>MNQETLIAVVEQMRKLVPALRKVPDETLYAWVEMAELFVCQKTFKDAYVKALALYALHLAFLDGALKGEDEDLESYSRRVTSFSLSGEFSQTFGEVTKNQSGDMMLSTPWGKMFEQLKARRRGRFALMTGLRGGCH[12x];>[12x]MKIVKHDGYNDIFNGGADGSPKPFFMSDASYHVGSFYNDNATAKRIVDVIPEEMVTAGFKMSGVKDEKEFKSLWDSYKLDSSLVDLLCWARLYGGAAMVAIIKDNRMLTSQAKPGAKLEGVRVYDRFAITVEKRVTNARSPRYGEPEIYKVSPGDNMQPYLIHHSRVFIADGERVAQQARKQNQGWGASVLNKSLIDAICDYDYCESLATQILRRKQQAVWKVKGLAEMCDDDDAQYAARLRLAQVDDNSGVGRAIGIDAETEEYDVLNSDISGVPEFLSSKMDRIVSLSGIHEIIIKNKNVGGVSASQNTALETFYKLVDRKREEDYRPLLEFLLPFIVDEEEWSIEFEPLSVPSKKEESEITKNNVESVTKAITEQIIDLEEARDTLRSIAPEFKLKDGNNINIREPEETTEPEPGLGEKLEDEN

Siphophage T1 is representative of the T series of model Escherichia coli phages, which has been observed to infect not only sensitive strains of E. coli but also some strains of Shigella dysenteriae. Siphophages possess a long, flexible, and non-contractile tail that plays a crucial role in host recognition, cell envelope penetration, and DNA injection. Connected to the head through a connector complex, the tail of a siphophage consists of three main components: a tail tube, a tape measure protein (TMP), and a distal tip. Using cryo-EM, we resolved the three-dimensional (3D) structures of the icosahedral head, head–tail complex and the tail tip of a laboratory-adapted fiberless mature T1 at resolutions of 3.5 Å, 3.6 Å, and 4.3 Å, respectively.

The T1 connector complex is composed of two dodecamers (a portal and an adaptor) and two hexamers (a stopper and a tail terminator). The density maps enable us to build the atomic models for the MCP gp47 and CPs (gp48 and gp49), connector complex (portal gp52, adaptor gp45, stopper gp44, and tail terminator gp42), and TTP gp41. In addition, the entire head–tail structure of T1 is also conserved compared with the widespread lambda-like members.>STNDNIKDLLDWYSSGSDTFTNSEVLDNSLGSMRIKNTDGSISLIIFPSPYYSPAFTKGEKVDLNTKRTKKSQHTSEGTYIHFQISGVTNTEKLPTPIELPLKVKVHGKDSPLKYWPKFDKKQLAISTLDFEIRAQLTQIHGLYRSSDKTGGYWKITMNDGSTYQ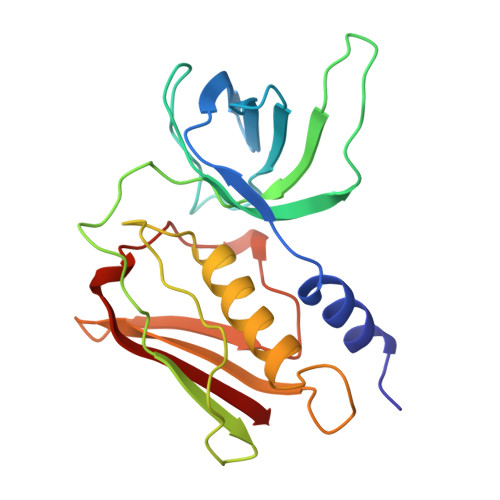SDLSKKFEYNTEKPPINIDEIKTIEAEIN[3x]>SNAVGLTPQDLSALTGVTRNLPKQLTQATQVAWSGPPPGFAKCPGGQVVILGFAMHLNFKEPGTDNFRIISCPPGREKCDGVGTASSETDEGRIYILCGEEPINEIQQVVAESPAHAGASVLEASCPDETVVVGGFGISVRGGSDGLDSFSIESCTTGQTICTKAPTRGSEKNFLWMMCVD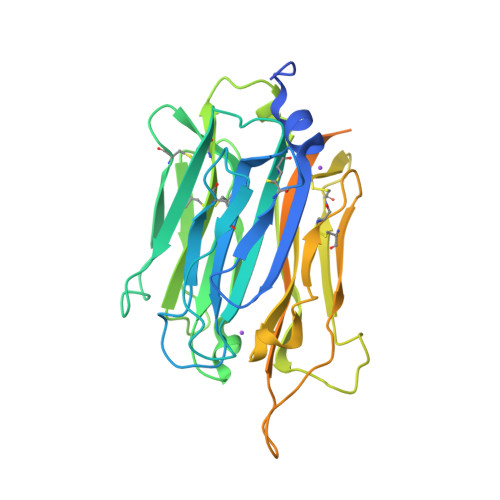KQYPGLRELVNVAELGSHGNANKRAVNSDGNVDVKCPANSSIVLGYVMEAHTNMQFVRDKFLQCPENASECKMTGKGVDHGMLWLFDRHALFGWIICKTVNEPAMHVATDVGKAKGNGKKKKGRKGKNKTNAPNEVEEGQQLGADSPSQVSVPADADSGPTSKTMSSLKLAPVKLLDL[2x]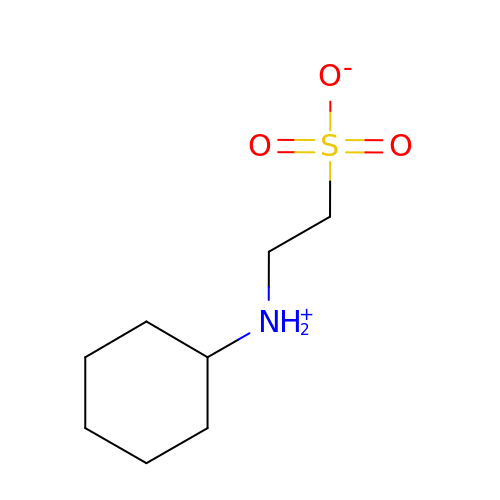2-(cyclohexylazaniumyl)ethanesulfonate | C8 H17 N O3 S | MKWKNSIESPFAQN-UHFFFAOYSA-N>MAEQVALSRTQVCGILREELFQGDAFHQSDTHIFIIMGASGDLAKKKIYPTIWWLFRDGLLPENTFIVGYARSRLTVADIRKQSEPFFKATPEEKLKLEDFFARNSYVAGQYDDAASYQRLNSHMNALHLGSQANRLFYLALPPTVYEAVTKNIHESCMSQIGWNRIIVEKPFGRDLQSSDRLSNHISSLFREDQIYRIDHYLGKEMVQNLMVLRFANRIFGPIWNRDNIACVILTFKEPFGTEGRGGYFDEFGIIRDVMQNHL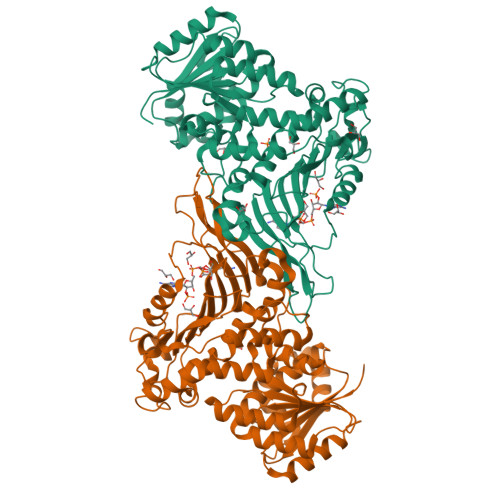LQMLCLVAMEKPASTNSDDVRDEKVKVLKCISEVQANNVVLGQYVGNPDGEGEATKGYLDDPTVPRGSTTATFAAVVLYVENERWDGVPFILRCGKALNERKAEVRLQFHDVAGDIFHQQCKRNELVIRVQPNEAVYTKMMTKKPGMFFNPEESELDLTYGNRYKNVKLPDAYERLILDVFCGSQMHFVRSDELLEAWRIFTPLLHQIELEKPKPIPYIYGSRGPTEADELMKRVGFQYEGTYKWVNPHKL[8x]>[4x]M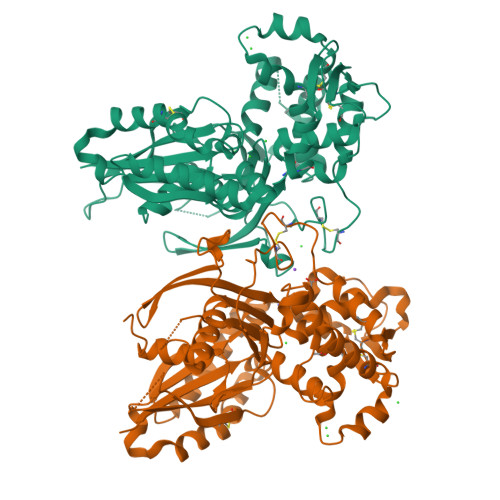AHHHHHHVGTGSNDDDDKSPDPTHNKPLPENVKYGIVLDAGSSHTNLYIYKWPAEKENDTGVVQQLEECQVKGPGISKYAQKTDEIAAYLAECMKMSTERIPASKQHQTPVYLGATAGMRLLRMESKQSADEVLAAVSRSLKSYPFDFQGAKIITGQEEGAYGWITINYLLGRFKTPGGSTFGALDLGGASTQITFVPLNSTLEAPETSLQFRLYGTDYTVYTHSFLCYGKDQALWQKLAQDIQVSSGGILKDPCFYPGYKKVVNVSELYGTPCTKRFEKKLPFNQFQVQGTGDYEQCHQSILKIFNNSHCPYSQCAFNGVFLPPLQGSFGAFSAFYFVMDFFKKMANDSVSSQEKMTEITKNFCSKPWEEVKASYPTVKEKYLSEYCFSGTYILSLLLQGYNFTGTSWDQIHFMGKIKDSNAGWTLGYMLNLTNMIPAEQPLSPPLPHST> SSQIRQNY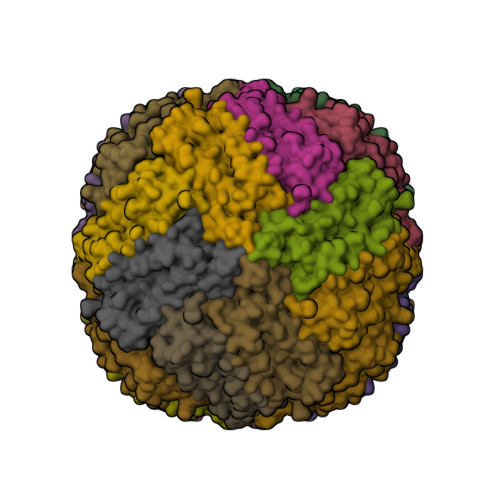STEVEAAVNRLVNLYLRASYTYLSLGFYFDRDDVALEGVCHFFRELAEEKMEGAERLLKMQNQRGGRALFQDLQKPSQDEWGTTPDAMKAAIVLEKSLNQALLDLHALGSAQADPHLCDFLESHFLDEEVKLIKKMGDHLTNIQRLVGSQAGLGEYLFERLTLKHD6-[ethyl-[3-(2-methylpropoxy)-4-propan-2-yl-phenyl]amino]pyridine-3-carboxylic acid | C21 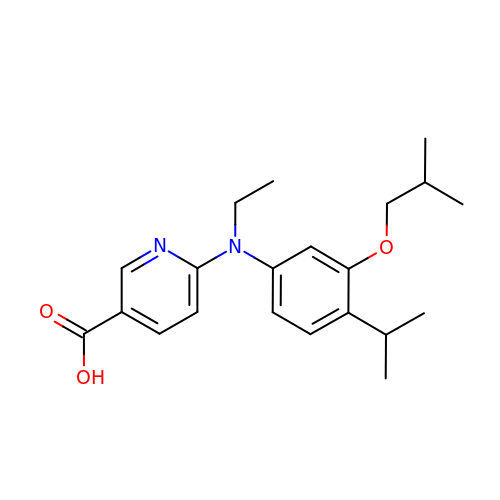H28 N2 O3 | JUCWZKDTWSKUAW-UHFFFAOYSA-N> PISPIETVPVKLKPGMDGPKVKQWPLTEEKIKALVEICTEMEKEGKISKIGPENPYNTPVFAIKKKDSTKWRKLVDFRELNKRTQDFWEVQLGIPHPAGLKKNKSVTVLDVGDAYFSVPLDEDFRKYTAFTIPSINNETPGIRYQYNVLPQGWKGSPAIFQSSMTKILEPFKKQNPDIVICQYMDDLYVGSDLEIGQHRTKIEELRQHLLRWGLTTPDKKHQKEPPFLWMGYELHPDKWTVQPIVLPEKDSWTVNDIQKLVGKLNWASQIYPGIKVRQLSKLLRGTKALTEVIPLTEEAELELAENREILKEPVHGVYYDPSKDLIAEIQKQGQGQWTYQIYQEPFKNLKTGKYARMRGAHTNDVKQLTEAVQKITTESIVIWGKTPKFKLPIQKETWETWWTEYWQATWIPEWEFVNTPPLVKLWYQLEKEPIVGAETFYVDGAANRETKLGKAGYVTNKGRQKVVPLTNTTNQKTELQAIYLALQDSGLEVNIVTDSQYALGIIQAQPDKSESELVNQIIEQLIKKEKVYLAWVPAHKGIGGNEQVDKLVSAGIRKIL;> PISPIETVPVKLKPGMDGPK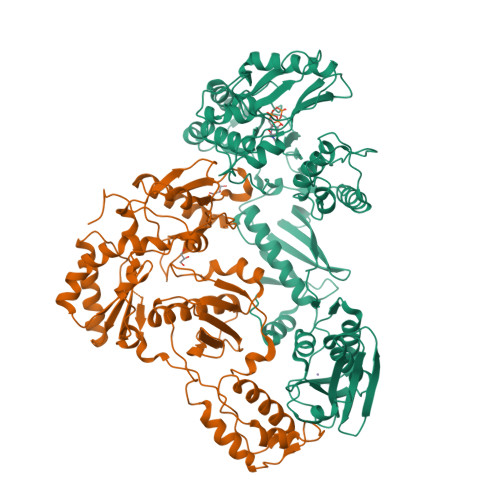VKQWPLTEEKIKALVEICTEMEKEGKISKIGPENPYNTPVFAIKKKDSTKWRKLVDFRELNKRTQDFWEVQLGIPHPAGLKKNKSVTVLDVGDAYFSVPLDEDFRKYTAFTIPSINNETPGIRYQYNVLPQGWKGSPAIFQSSMTKILEPFKKQNPDIVICQYMDDLYVGSDLEIGQHRTKIEELRQHLLRWGLTTPDKKHQKEPPFLWMGYELHPDKWTVQPIVLPEKDSWTVNDIQKLVGKLNWASQIYPGIKVRQLSKLLRGTKALTEVIPLTEEAELELAENREILKEPVHGVYYDPSKDLIAEIQKQGQGQWTYQIYQEPFKNLKTGKYARMRGAHTNDVKQLTEAVQKITTESIVIWGKTPKFKLPIQKETWETWWTEYWQATWIPEWEFVNTPPLVKLWYQLEKEPIVGAETFYVDGAAN>MTELPIDENTPRILIVEDEPKLGQLLIDYLRAASYAPTLISHGDQVLPYVRQTPPDLILLDLMLPGTDGLMLCREIRRFSDIPIVMVTAKIEEIDRLLGLEIGADDYICKPYSPREVVARVKTILRRCKPQRELQQQDAESPLIIDEGRFQASWRGKMLDLTPAEFRLLKTLSHEPGKVFSREQLLNHLYDDYRVVTDRTIDSHIKNLRRKLESLDAE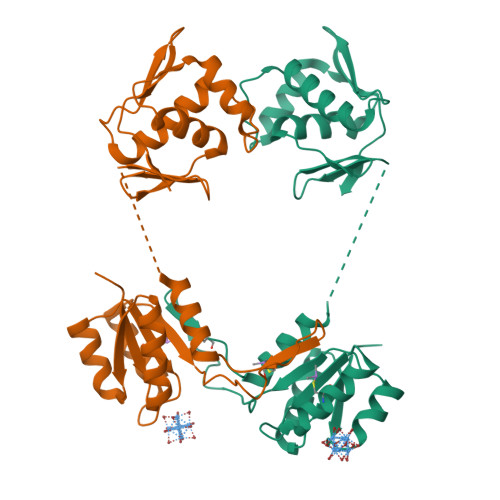QSFIRAVYGVGYRWEADACRIV[12x]N-(SULFANYLACETYL)TYROSYLPROLYLMETHIONINAMIDE | C21 H30 N4 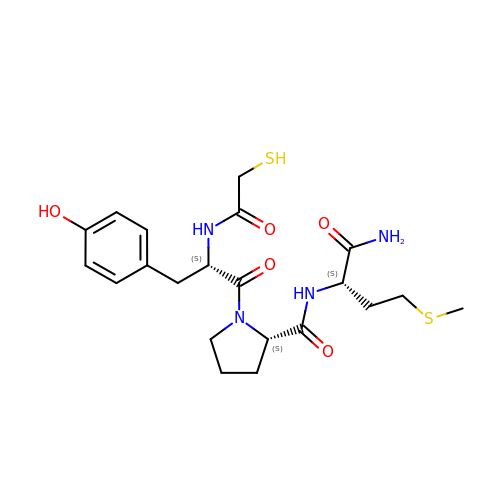O5 S2 | LNLWXWOYQHAKTD-ULQDDVLXSA-N> TDW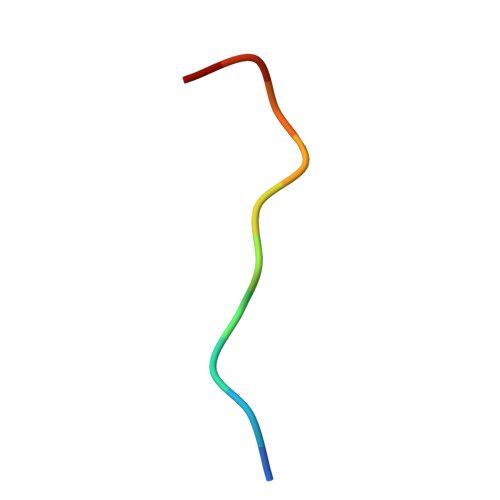VDPSFDDF> GAMFQIKARPYERFADVEKPWIQKHSMDSKLVPANKGNLIQAEIVYQSVSEHSDLVISPVNEIRPANRFPSHRKSFFAENLRASPPVVPVAVDKYAVPVANPMDPENPNAWDVTLKITTKAVTVPVDVVMVIDQSSSMGGQNIARLKSAIASGQRFVKKMLPKGMATEGVRIALVSYDHEPHRLSDFTKDTAFLCQKIRALTPIWGTHTQGGLKMARNIMATSTAVDKHIILMSDGLATEQYPVKNVTTADFIGETGNANDPIDLVIQGAINFPTNYVSNNPSTPLTPNYPTHSSKVGRRNLPESKFDYSNLSARITFDGVAGALVYEPRFPHPYYYYFPCNAAINEAQFAKNSGYTIHTIGYDLGDFALANNSLKLTATDENHFFTATPANLAAAFDNIAQTINIGIQRGEVTDFVAPGFIVKNLTQSGDVTHLLNVSNGTVHYDVSTKKLTWTTGTILSSSEATITYRIYADLDYIQNNDIPVNTTSAIGPDLGGFDTNTEAKLTYTNSNGESNQQLIFPRPTVKLGYGVIKRHYVLVNKDGQPIQANGTVVSSLSEAHVLQSQDFFLPSGGGHIVPKWIKLDKTTEALQYYSVPPTNTVITTADGKRYRFVEVPGSTPNPGQIGISWKKPAGNAYFAYKLLNYWMGGTTDQQSEWDVTSNWTGAQVPLTGEDVEFATTENFGSPAVADLHVPTTNPKIIGNLINNSDKDLVVTTNSQLTINGVVEDNNPNVGTIVVKSSKDNPTGTLLFANPGYNQNVGGTVEFYNQGYDCADCGMYRRSWQYFGIPVNESGFPINDVGGNETVNQWVEPFNGDKWRPAPYAPDTKLQKFKGYQITNDVQAQPTGVYSFKGTLCVCDAFLNLTRTSGVNYSGANLIGNSYTGAIDIKQGIVFPPEVEQTVYLFNTGTRDQWRKLNGSTVSGFRAGQYLSVPKNTAGQDNLPDRIPSMHSFLVKMQNGASCTLQILYDKLLKNTTVNNGNGTQITWRSGNSGSANMPSL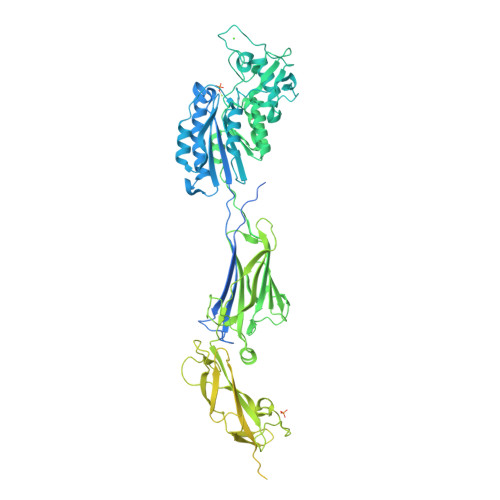VMDVLGNESADRLWIFTDGGLSFGFD 1a,20S-dihydroxyvitamin D3 | C27 H44 O3 | 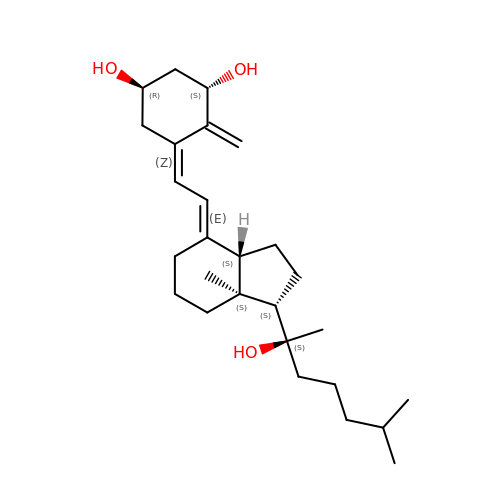RLDKSDBKVGPMKA-YAUUYYILSA-N> MTSLRDLIPKHKFDNSTIDQLC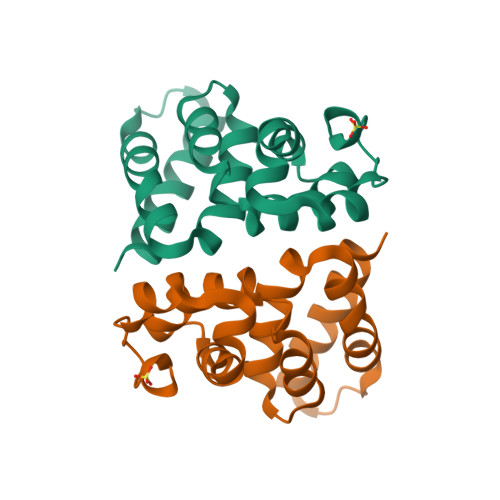KLIDNEIEPIIFDLLKWLQDYNWPIAKDILPVVVLHQSIAMPHILTILQGNDIMWKYWVIKLMIPYLIYPNKQLVKSELERLSSLEIINEDIREIVNLSKDYLHFYYP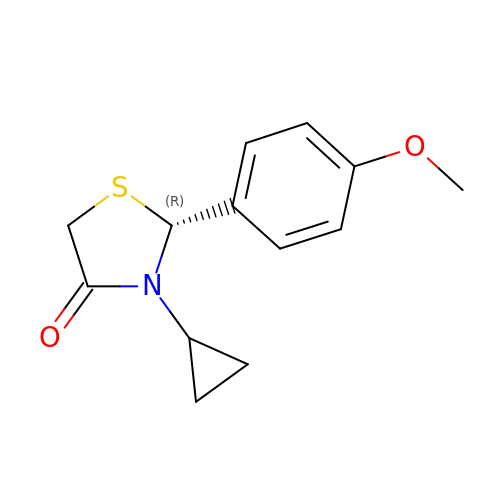(2R)-3-cyclopropyl-2-(4-methoxyphenyl)-1,3-thiazolidin-4-one | C13 H15 N O2 S | LFCBYPLPSCPFNK-CYBMUJFWSA-N3-[(3,5-dimethyl-1,2-oxazol-4-yl)methyl]-5-methyl-1,3,4-thiadiazol-2(3H)-one 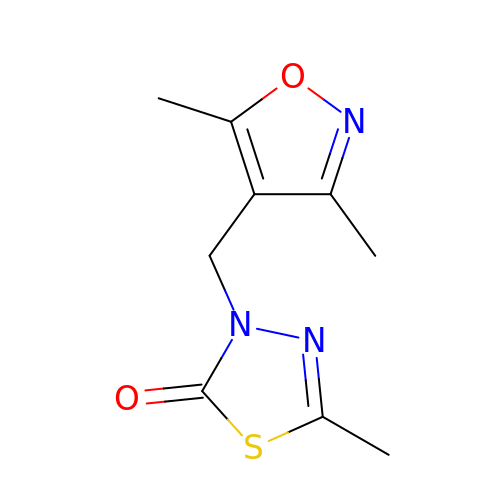| C9 H11 N3 O2 S | QMZRSGJUZDOFDN-UHFFFAOYSA-N>MLSKVKKVPSPYVGNLLNKWHDYIMQEKVHESIEKRTEIKQLLSQAEDNKDLVDYFILLDHRHSLCFDQEASMGDVVNMLSKGSHDLLINFYFELFAGDYEFFKKNYVKAISFYEKAEQKLSSIPNIEETKFAEFHYKIGVAYYEIDQHLVSVNKVTKARDIYKKSDMWNLEAIQCSLVVGINLYDMGRLDDADAYFRDALTEALDHGYDKPITKIYHNLGLVHWQKGSLELALHYFREAYSHEWLRDSPKGQQTVYMLSRVLYTMGQNEEAYHWYELGIEMARKFDDHEYKAKHDILYHLYE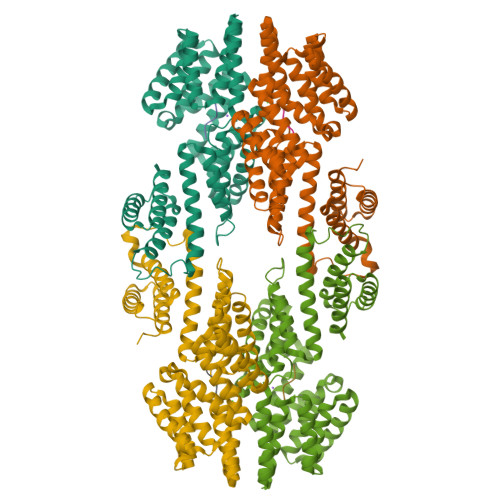QPSIDEVKQSLAFLEERNLWPDVSKIAKGISELYEKKGDLVTSHEFLKRAFYAKEQIQRITEALGLEHHHHHH[4x];>[4x]MKKINGWIVVALLAVTTVGAAAAIQYTNNADSPGQFQVAQKGMY> MPPAIVVLIGPPGYVGKQYPITASDIVIGRSVESQVYIDDKSLS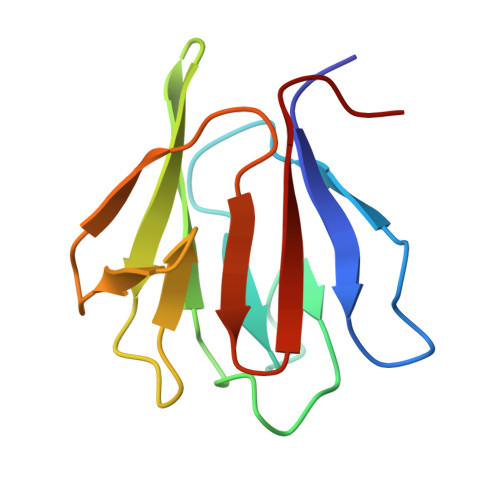RSHAKFAVNGSEVSVIDLGSTNKTIVNGQVIPPLASCLLKNNDQIKTGNVIFKFLEKGS> MLSETELRALKKLSTTTSRVVGDSTLALPSNVKLSKGEVEKIAVTKKEMFDELAQCNLPTIELITREHTFNGDVIRFAAWLFLMNGQKLMIANNVAVRMGMQYATNLAGNNVKITYVTSNNVVKLGHIAAGVLANPYSNKGSGLFITYEYNLISNLIETGKVCVLFITSLSTTASSTNSFAYSTCSVPIENWDFNMIKLTAETSCASLTAMTNLVNSL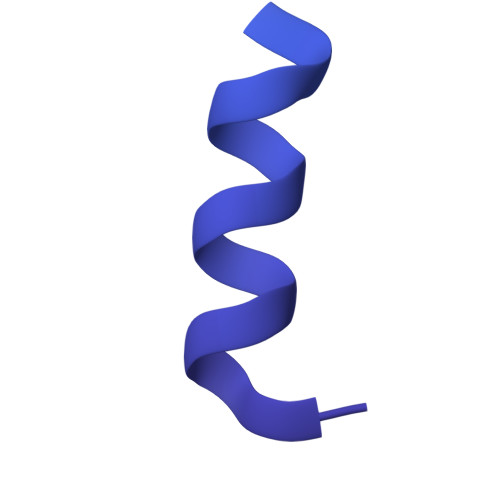VPGERTRPVGLYVDIPGVTVTTSASSGSLPLTTIPAVTPLIFSAYTKQVEEVGVINTLYALSYLP> NREKDCSSSSEVESQSKCRKESTAEPDSLSRDT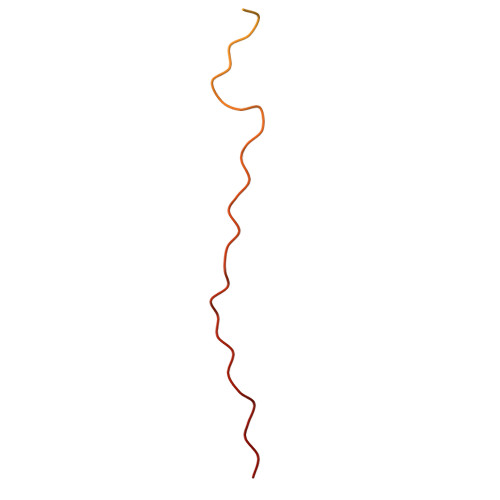RTTSSLKSSTSFPISFKGSIDLKSLNQPSSLLHIQVSPTKSSNLDAQVNTEQAYSQPFRY>[8x]GSHMPGQQATKHESLLDQLSLKGKVVVVTGASGPKGMGIEAARGCAEMGAAVAITYASRAQGAEENVKELEKTYGIKAKAYKCQVDSYESCEKLVKDVVADFGQIDAFIANAGATADSGILDGSVEAWNHVVQVDLNGTFHCAKAVGHHFKERGTGSLVITASMSGHIANFPQEQTSYNVAKAGCIHMARSLANEWRDFARVNSISPGYIDTGLSDFVPK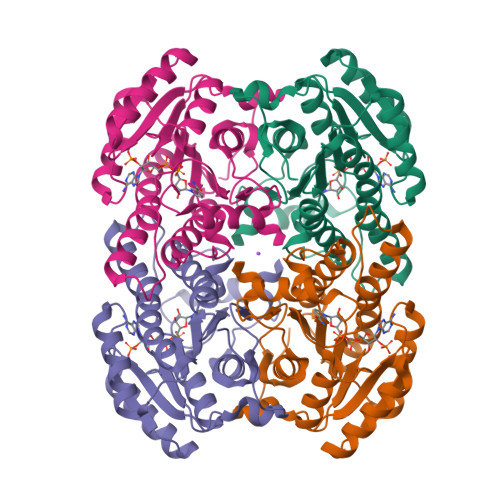ETQQLWHSMIPMGRDGLAKELKGAYVYFASDASTYTTGADLLIDGGYTTR> VEATAQETDRPRFSFSIAA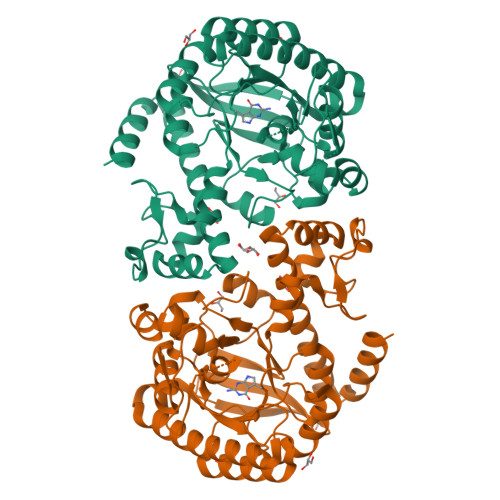REGKARTGTIEMKRGVIRTPAFMPVGTAATVKALKPETVRATGADIILGNTYHLMLRPGAERIAKLGGLHSFMGWDRPILTDSGGFQVMSLSSLTKQSEEGVTFKSHLDGSRHMLSPERSIEIQHLLGSDIVMAFDECTPYPATPSRAASSMERSMRWAKRSRDAFDSRKEQAENAALFGIQQGSVFENLRQQSADALAEIGFDGYAVGGLAGGEGQDEMFRVLDFSVPMLPDDKPHYLMGVGKPDDIVGAVERGIDMFDCVLPTRSGRNGQAFTWDGPINIRNARFSEDLKPLDSECHCAVCQKWSRAYIHHLIRAGEILGAMLMTEHNIAFYQQLMQKIRDSISEGRFSQFAQDFRARYFARNS> GHMERLLDELTLEGVARYMQSERCRRVICLVGAGISTSAGIPDFRSPSTGLYDNLEKYHLPYPEAIFEISYFKKHPEPFFALAKELYPGQFKPTICHYFMRLLKDKGLLLRCYTQNIDTLERIAGLEQEDLVEAHGTFYTSHCVSASCRHEYPLSWMKEKIFSEVTPKCEDCQSLVKPDIVFFGESLPARFFSCMQSDFLKVDLLLVMGTSLQVQPFASLISKAPLSTPRLLINKEKAGQSDPFLGMIMGLGGGMDFDSKKAYRDVAWLGECDQGCLALAELLGWKKELEDLVRREHASIDAQS;> EALPKATGG

Sirtuins (SIRTs) are nicotinamide adenine dinucleotide (NAD+)‐dependent lysine deacylases linked to key physiological and disease processes. SIRTs catalyze lysine deacylation through a distinctive mechanism in which the amide oxygen of the acylated lysine transiently attacks the C1’ of the nicotinamide riboside residue from NAD+ (hereafter referred to as C1’ of NAD+ ribose), forming a covalent ADP‐ribosylated intermediate. Here, we report a new class of mechanism‐based 1,2,3‐triazole inhibitors that hijack SIRT catalysis by forming stalled triazolium– or triazole–ADP‐ribose (ADPR) adducts derived from the cofactor NAD+. These trapped adducts inhibit the enzyme without covalent protein modification, prompting us to term the compounds “Sirtuin Trapping Ligands” (SirTraps).

Compounds OTi‐1 (3, ornithine‐triazolyl inhibitor 1) and LTi‐1 (4, lysine‐triazolyl inhibitor 1) mimic acetylated lysine (Kac), whereas OTDi‐1 (5, ornithine‐triazolyl‐dodecyl inhibitor 1) and LTDi‐1 (6, lysine‐triazolyl‐dodecyl inhibitor 1) mimic Kmyr through their dodecyl extensions, engaging the full acyl‐lysine channel. To elucidate the molecular basis of this unexpected mode of inhibition, co‐crystallization experiments were performed with SIRT2 and compounds 5 and 6, both in the absence and presence of NAD⁺. In contrast, significant melting temperature shifts were observed for 5 and 6 at 10 µM, further enhanced by NAD+ addition (ΔT m: 5 = 9.9 ± 0.0 °C, 6 = 16.3 ± 0.1 °C), indicating strong SIRT2 stabilization. While NAD+ preincubation also improved the affinity of compound 5 (IC50 = 0.76 ± 0.25 µM), its potency remained > 200‐fold lower than for 6. In contrast, 5 needs to adopt a deeper position, leading to suboptimal geometry and too close contacts with the acyl‐lysine channel entrance (Phe235–Leu239).> MGSSHHHHHHLEVLFQGPHMASKYIIEHMEEGFSEWVILEYSQILREVGAENLILSSLPESTTEKDIPQRLLKLGLRWTTKDLKGINEDFKDLELLKDGRVCLLDPRATIDLQPEDATKFDYFVFGGILGDHPPR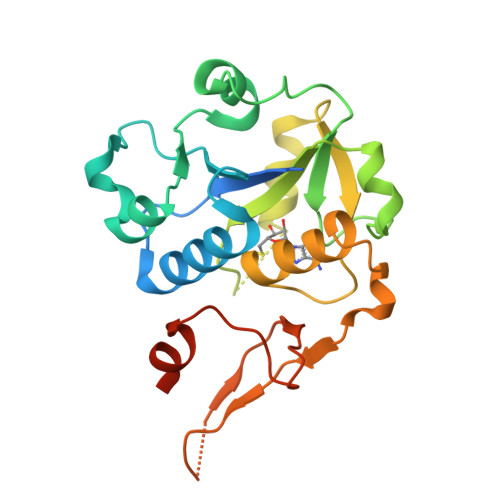DRTKELKTAYPNLLISRRLGDKQMTTDTAIRTTQLIIKDRIAFEDIKFIDYPEFRFNKNEATEMPFRYVLDKEGKPILPEGMLDLIKKDSAQSLDDLLM>[3x]HSMHHHHHHLGNKLSISDLKDIKNKKVLVRVDFNVPIENGIIKDTNRITATLPTINHLKKEGASKIILISHCGRPDGLRNEKYTLKPVAETLKGLLGEEVLFLNDCVGKEVEDKINA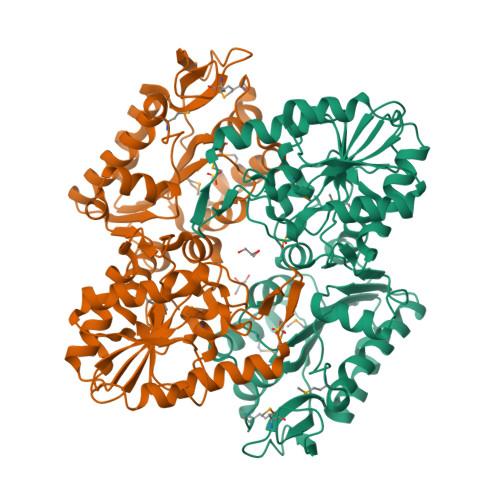AKENSVILLENLRFHIEEEGKGVDANGNKVKANKEDVEKFQNDLTKLADVFINDAFGTAHRAHSSMVGVKLNVKASGFLMKKELEYFSKALENPQRPLLAILGGAKVSDKIQLIKNLLDKVDRMIIGGGMAYTFKKVLNNMKIGTSLFDEAGSKIVGEIMEKAKAKNVQIFLPVDFKIADNFDNNANTKFVTDEEGIPDNWMGLDAGPKSIENYKDVILTSKTVIWNGPQGVFEMPNFAKGSIECLNLVVEVTKKGAITIVGGGDTASLVEQQNKKNEISHVSTGGGASLELLEGKELPGVLALSNK>MKELIRKLTEAFGPSGREEEVRSIILEELEGHIDGHRIDGLGNLIVWKGSGEKKVILDAHIDEIGVVVTNVDDKGFLTIEPVGGVSPYMLLGKRIRFENGTIGVVGMEGETTEERQENVRKLSFDKLFIDIGANSREEAQKMCPIGSFGVYDSGFVEVSGKYVSKAMDDRIGCAVIVEVFKRIKPAVTLYGVFSVQEEVGLVGASVAGYGVPADEAIAIDVTDSADTPKAIKRHAMRLSGGPALKVKDRASISSKRILENLIEIAEKFDIKYQMEVLTFGGTNAMGYQRTREGIPSATV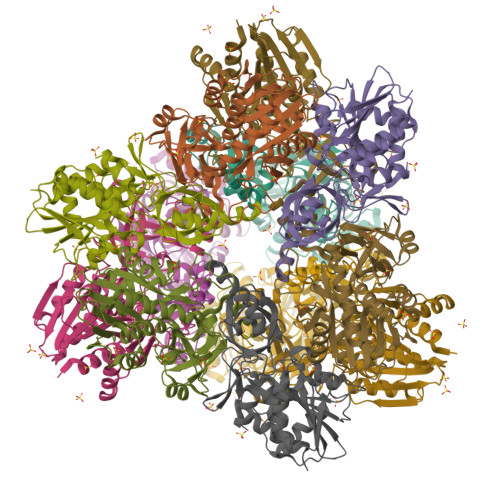SIPTRYVHSPSEMIAPDDVEATVDLLIRYLGA[4x]>[2x]MVQPSLPQDDTPDQQEQRNRAIAQQREAYQYSETAGILLIKTLPQSEMFSLKYLIERDKGLVSLIANTLASNIENIFDPFDKLEDFEEMFPLLPKPLVMNTFRNDRVFARQRIAGPNPMVIERVVDKLPDNFPVTDAMFQKIMFTKKTLAEAIAQGKLFITNYKGLAELSPGRYEYQKNGTLVQKTKTIAAPLVLYAWKPEG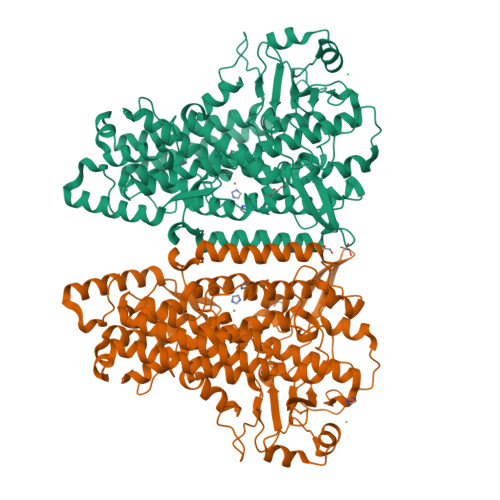FGDYRGSLAPIAIQINQQPDPITNPIYTPRDGKHWFIAKIFAQMADGNCHEAISHLARTHLILEPFVLATANELAPNHPLSVLLKPHFQFTLAINELAREQFISAGGYADDLLAGTLEASIAVIKAAIKEYMDNFTEFALPRELARRGVGIGDVDQRGENFLPDYPYRDDAMLLWNAIEVYVRDYLSLYYQSPVQIRQDTELQNWVRRLVSPEGGRVTGLVSNGELNTIEALVAIATQVIFVSGPQHAAVNYPQYDYMAFIPNMPLATYATPPNKESNISEATILNILPPQKLAARQLELMRTLCVFYPNRLGYPDTEFVDVRAQQVLHQFQERLQEIEQRIVLCNEKRLEPYTYLLPSNVPNSTSI N-[2-fluoro-4-(4-phenylpiperidine-1-sulfonyl)benzoyl]glycine 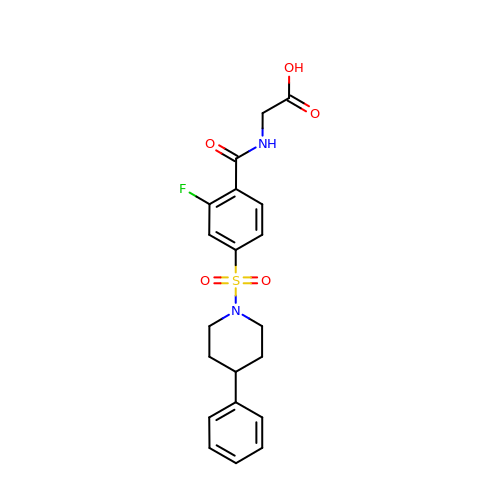| C20 H21 F N2 O5 S | IOUTWRYTULEKGO-UHFFFAOYSA-N>[2x]MTGSEIFLASKRAAITYDTDPATGEPRAWLAPGGTGNVVAEQAGVLNISWIASADSEDDRRASALNPDGVTMELHSGREILVRLIR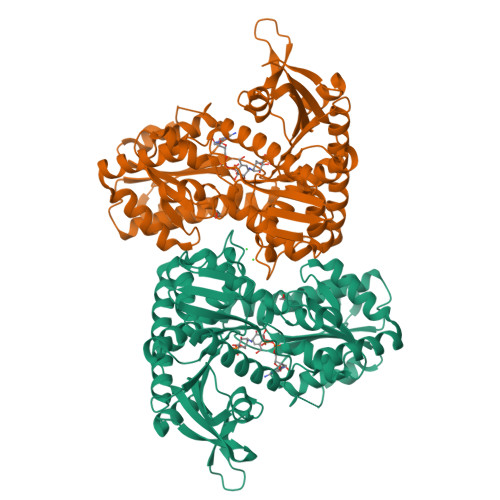HDPAVFRNVQNFMTANLMWAANNYGWDRWTQPSFGSDAREGWADFGRFTRDFADAILKSSAQSADPVYLVHDYQLVGVPALLREQRPDAPILLFVHIPWPSADYWRILPKEIRTGILHGMLPATTIGFFADRWCRNFLESVADLLPDARIDREAMTVEWRGHRTRLRTMPLGYSPLTLDGRNPQLPEGIEEWADGHRLVVHSGRTDPIKNAERAVRAFVLAARGGGLEKTRMLVRMNPNRLYVPANADYVHRVETAVAEANAELGSDTVRIDNDNDVNHTIACFRRADLLIFNSTVDGQNLSTFEAPLVNERDADVILSETCGAAEVLGEYCRSVNPFDLVEQAEAISAALAAGPRQRAEAAARRRDAARPWTLEAWVQAQLDGLAADHAARTATAERFDTAPAVSTRADL>GGGGGGMLNRVFLEGEIESSCWSVKKTGFLVTIKQMRFFGERLFTDYYVIYANGQLAYELEKHTKKYKTISIEGILRTYLERKSEIWKTTIEIVKIFNPKNEIVI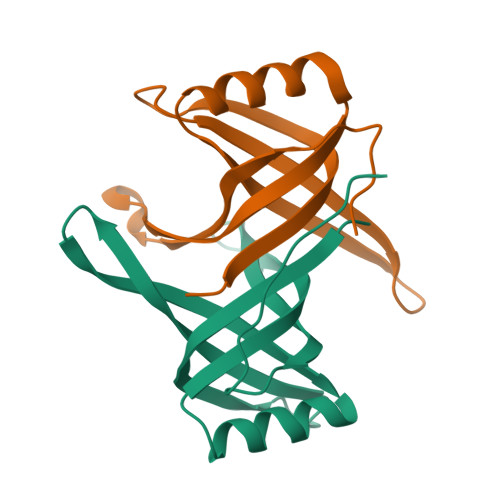DYKEI[6x]> MGSSHSSGLVPRGSMKNDRTLQAIGRQLKAMGCERFDIGVRDATTGQMMNREWSAAEVLQNTPWLKRMNAQGNDVYIRPAEQERH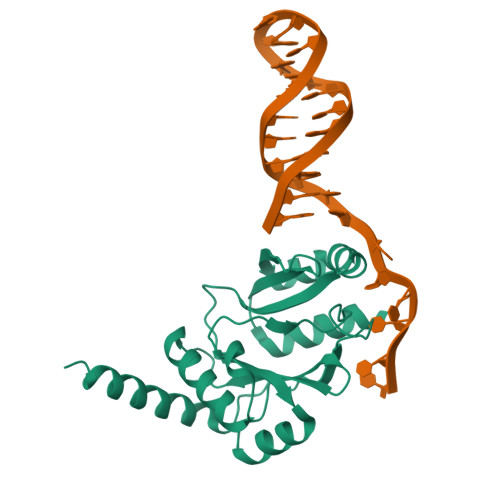GLVLVDDLSEFDLDDMKAEGREPALVVETSPKNYQAWVKVADAAGGELRGQIARTLASEYDADPASADSRHYGRLAGFTNRKDKHTTRAGYQPWVLLRESKGKTATAGPALVQQAGQQIEQAQRQQEKARRLASLELPERQ>[4x]MGMSSIGLAHNVTILGSGETTVVLGHGYGTDQSVWKLLVPYLVDDYKVLLYDHMGAGTTNPDYFDFDRYSSLEGYSYDLIAILEEFQVSKCIYVGHSMSSMAAAVASIFRPDLFHKLVMISPTPRLINTEEYYGGFEQKVMDETLR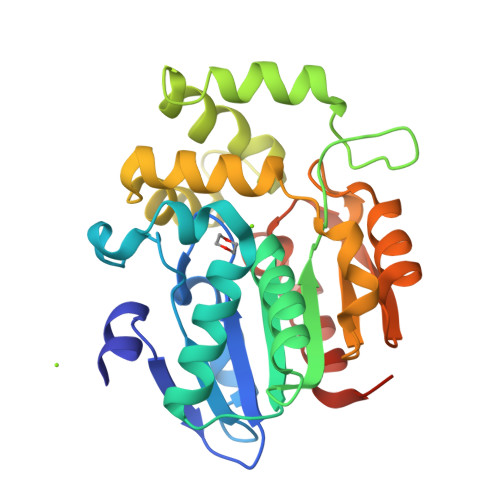SLDENFKSLSLGTAPLLLACDLESAAMQEYCRTLFNMRPDIACCITRMICGLDLRPYLGHVTVPCHIIQSSNDIMVPVAVGEYLRKNLGGPSVVEVMPTEGHLPHLSMPEVTIPVVLRHIRQDITDHTRHHHHHH>[2x]SQEVMKNLSL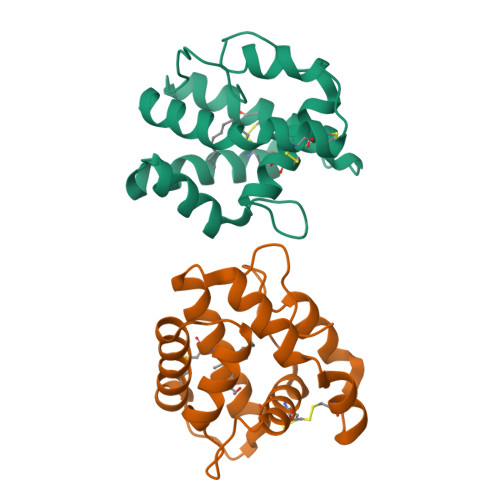NFGKALDECKKEMTLTDAINEDFYNFWKEGYEIKNRETGCAIMCLSTKLNMLDPEGNLHHGNAMEFAKKHGADETMAQQLIDIVHGCEKSTPANDDKCIWTLGVATCFKAEIHKLNWAPSMDVAVGE>MSNKYRVRKNVLHLTDTEKRDFVRTVLILKEKGIYDRYIAWHGAAGKFHTPPGSDRNAAHMSSAFLPWHREYLLRFERDLQSINPEVTLPYWEWETDAQMQD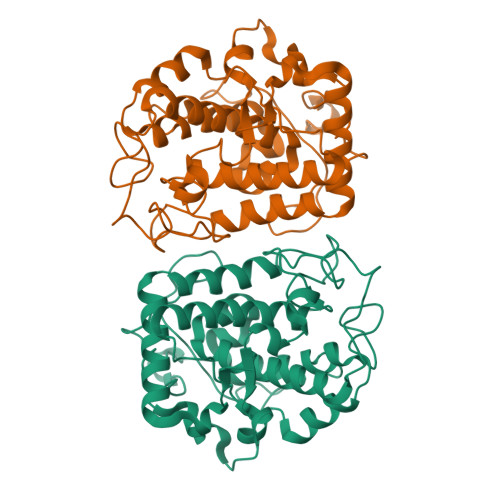PSQSQIWSADFMGGNGNPIKDFIVDTGPFAAGRWTTIDEQGNPSGGLKRNFGATKEAPTLPTRDDVLNALKITQYDTPPWDMTSQNSFRNQLEGFINGPQLHNRVHRWVGGQMGVVPTAPNDPVFFLHHANVDRIWAVWQIIHRNQNYQPMKNGPFGQNFRDPMYPWNTTPEDVMNHRKLGYVYDIELEKSKRSSHHHHHH[2x]In the presence of NADH, acetoin is reduced to 2,3-BDO by the enzyme butanediol dehydrogenase (Bdh). SmBdh exhibits the typical single domain short-chain dehydrogenase/reductase (SDR) architecture. A monomer displays a dinucleotide-binding Rossmann fold that includes seven-stranded parallel β-sheet (β3–β2–β1–β4–β5–β6–β7) flanked by three α-helices (α2, α1, and α8) on one side and three α-helices (α3, α4, and α5) on another. There is an additional small lobe on top of a core structure, formed by two short helices, α6 and α7, creating a deep cleft in which the cofactor is bound, and where the active site is located.

The Z. mobilis expressed WT SmBdh crystallized in the space group P43212 with two protein molecules per asymmetric unit that could be superimposed with r.m.s.d. of 0.271 Å over 1379 atoms. Two molecules found in the asymmetric unit form a tetramer (dimer of dimers) with a symmetry-related dimer with extensive interface surfaces. The main difference between the two molecules in the asymmetric unit is that molecule A is found in ‘closed’ conformation (that could be best described by ~ 10 Å distance between Cα-atoms of residues Ala93 and Trp192) and molecule B is found in ‘open’ conformation (the same distance is ~ 14 Å). The transition from the ‘open’ conformation into the ‘closed’ seems to be coincidental with NAD + binding and includes the shift of the loop 183–203, containing two helices, α6 and α7. WT SmBdh contains acetoin in the substrate-binding pocket of the ‘closed’ molecule A. Crystallization conditions included NAD + and acetoin, and more acetoin was used for cryoprotection. We interpreted this as both (3R)- and (3S)-acetoin molecules bound in the pocket since commercially available acetoin is a racemic mixture and no other small molecules (like ethylene glycol) were added during crystallization or as a cryoprotectant. Whereas the positions of all acetoin atoms, with the exception of O3, superimpose quite well; the O3 atoms of (3S)- and (3R)-acetoin molecules are involved in hydrogen bonds with different surrounding residues. In contrast, O3 atom of the (3R)-acetoin has three possible partners for H-bond formation: water molecule W71 (2.7 Å), Nε of the Gln247symm (3.1 Å), and Ser140Oγ (3.1 Å). We found that the substrate-binding pocket is formed by two protein molecules, not a single peptide as found in all other reported Bdh enzymes. The side chain of Q247symm is involved in the substrate positioning forming a hydrogen bond with the O3 atom of the acetoin.

>[2x]MHHHHHHENLYFQGRFDNKVVVITGAGNGMGEAAARRFSAEGAIVVLADWAKEAVDKVAASLPKGRAMAVHIDVSDHVAVEKMMNEVAEKLGRIDVLLNNAGVHVAGSVLETSIDDWRRIAGVDIDGVVFCSKFALPHLLKTKGCIVNTASVSGLGGDWGAAYYCAAKGAVVNLTRAMALDHGGDGVRINSVCPSLVKTNMTNGWPQEIRDKFNERIALGRAAEPEEVAAVMAFLASDDASFINGANIPVDGGATASDGQPKIV ethyl 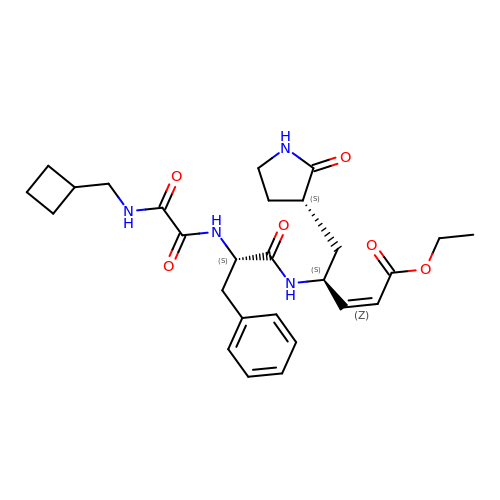(2Z,4S)-4-[(N-{[(cyclobutylmethyl)amino](oxo)acetyl}-L-phenylalanyl)amino]-5-[(3S)-2-oxopyrrolidin-3-yl]pent-2-enoate | C27 H36 N4 O6 | JXIYUFBHNQDFQS-BDTNDASRSA-N> ADAPFEGRKKCSSCHKAQAQSWKDTAHAKAMESLKPNVKKEAKQKAKLDPAKDYTQDKDCVGCHVDGFGQKGGYTIESPKPMLTGVGCESCHGPGRNFRGDHRKSGQAFEKSGKKTPRKDLAKKGQDFHFEERCSACHLNYEGSPWKGAKAPYTPFTPEVDAKYTF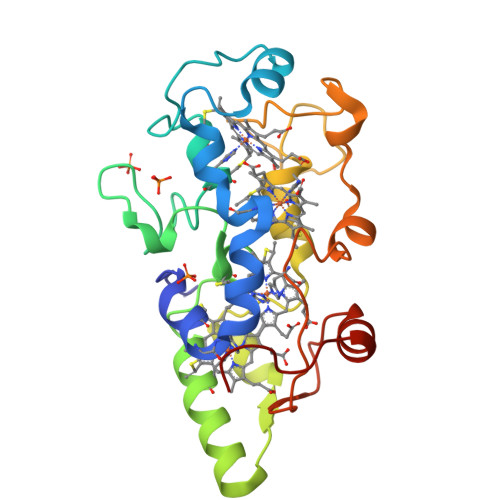KFDEMVKEVKAMHEHYKLEGVFEGEPKFKFHDEFQASAKPAKKGK> GSNECISVKGRIYSILKQIGSGGSSKVFQVLNEKKQIYAIKYVNLEEADNQTLDSYRNEIAYLNKLQQHSDKIIRLYDYEITDQYIYMVMECGNIDLNSWLKKKKSIDPWERKSYWKNMLEAVHTIHQHGIVHSDLKPANFLIVDGMLKLIDFGIANQMQPDTTSVVKDSQVGTVNYMPPEAIKDMSSSRENGKSKSKISPKSDVWSLGCILYYMTYGKTPFQQIINQISKLHAIIDPNHEIEFPDIPEKDLQDVLKCCLKRDPKQRISIPELLAHPYV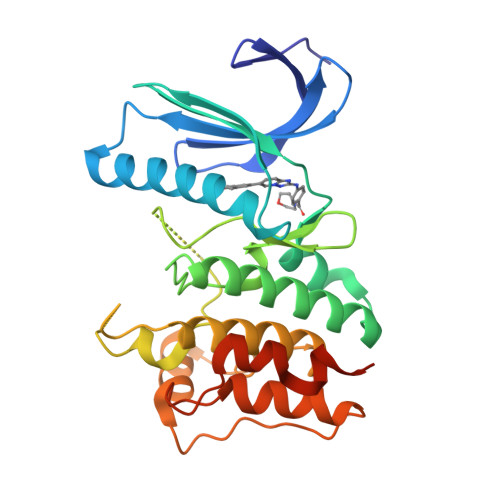QIQTHPVNQMAKGTT> AGAQDFVPHTADLAELAAAAGECRGCGLYRDATQAVFGAGGRSARIMMIGEQPGDKEDLAGLPFVGPAGRLLDRALEAADIDRDALYVTNAVKHFKFTRAAGGKRRIKKTPSRTEVVACRPWLIAEMTSVEPDVVVLLGATAAKALLGNDFRVTQHRGEVLHVDDVPGDPALVATVHPSSLLRGPKEERESAFAGLVDDLRVAADV

UdgX excises uracil from uracil-containing DNA to concurrently form a covalent bond with the resulting AP-DNA. Structurally, UdgX is highly similar to family-4 UDGs (F4-UDGs). However, UdgX is unique in possessing a flexible R-loop (105KRRIH109). Our earlier studies allowed us to propose a reaction mechanism of UdgX, which involves the formation of a covalent bond between H109 of UdgX with the C1′ position of the target deoxyribose sugar concurrently with the uracil excision from this site in DNA.

Substitutions of His109 in MsmUdgX with Ser, Gly, Ala, Gln, Cys and Lys showed the loss of its covalent complex formation with DNA but gained canonical UDG activities. In the reactions of the mutant proteins with ssU9, the entire substrate was converted to product by the H109G mutant, while hardly any substrate was utilized by the H109K mutant. However, H109 substitutions by Gln or Lys, showed poor activity. However, to better understand the mechanism of uracil excision by the H109 mutants, we determined their structures along with a pentameric DNA, TTUTT by X-ray crystallography. The DNA backbone could not be modelled into the experimental electron density map in any of the mutant structures that were determined. Nonetheless, all structures revealed the excised uracil and the side chain substitutions at position 109. The structures also revealed invariant interactions of N91 and H178 with uracil. When we arranged the mutants in the order of increasing cavity sizes (left), we noted that the canonical UDG activity of the mutants increased with their increasing cavity sizes to begin with and then with a further increase in the cavity size, the UDG activity declined (right). It suggested that the initial increase in UDG activity (H109K to H109Q to H109G) occurred because of the efficiency with which the water molecule could be localized to make a nucleophilic attack on the C1′ position.>[2x]QANTSYTDYNVEANPDLFPLCLQHLNASFPDCASGPLSLTPVCDRSLSPKDRATALVSLFTFDELVNNTGNTGLGVSRLGLPNYQVWGEALHGVGRANFVESGNFSWATSFPMPITMMAALNKTLIHQIGTIVSTQLRAFSNAGLGGVDVYSPNINTFRHPVWGRGQETPGEDAFLTSVYGYEYITALQGGVDPETLKIIATAKHYAGYDIESWNNHSRLGNDMQITQQELSEYYTPPFIVASRDAKVRSVMCSYNAVNGVPSCANKFFLQTLLRDTFEFSEDGYVSGDCGAVYNVWNPHGYASNEAAASADSILAGTDIDCGTSYQWHSEDAFEDSLVSRSDIERGVIRLYSNLVQAGYFDGEDAPYRDITWDDVLSTDAWNIAYEAAVEGIVLLKNDETLPLSKDIKSVAVIGPWA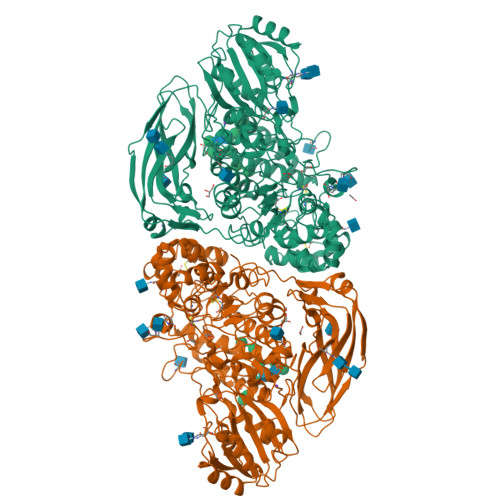NVTEELQGNYFGPAPYLISPLTGFRDSGLDVHYALGTNLTSHSTSGFEEALTAAKQADAIIFAGGIDNTIEAEAMDRENITWPGNQLDLISKLSELGKPLVVLQMGGGQVDSSSLKDNDNVNALIWGGYPGQSGGHALADIITGKRAPAGRLVTTQYPAEYAEVFPAIDMNLRPNETSGNPGQTYMWYTGTPVYEFGHGLFYTTFEESTETTDAGSFNIQTVLTTPHSGYEHAQQKTLLNFTATVKNTGERESDYTALVYVNTTAGPAPYPKKWVVGFDRLGGLEPGDSQTLTVPVTVESVARTDEQGNRVLYPGSYELALNNERSVVVKFELKGEEAVILSWPEDTTSDFVSSIDGGLDRKQDVIA> MAGSREILLPEVHLNSPIVKHKLYYYILLGNLPNEIDLDDLGPLHNQNWNQIAHEESNLAQRLVNVRNFLITHIPDLRKGHWQEYVNVILWPRILPLIPDFKINDQLPLLKNWDKLVKESCSVINAGTSQCIQNLSYGLTGRGNLFTRSRELSGDRRDIDLKTVVAAWHDSDWKRISDFWIMIKFQMRQLIVRQTDHNDSDLITYIENREGIIIITPELVALFNTENHTLTYMTFEIVLMVSDMYEGRHNILSLCTVSTYLNPLKKRITYLLSLVDNLAFQIGDAVYNIIALLESFVYAQLQMSDPIPELRGQFHAFVCSEILDALRGTNSFTQDELRTVTTNLISPFQDLTPDLTAELLCIMRLWGHPMLTASQAAGKVRESMCAGKVLDFPTIMKTLAFFHTILINGYRRKHHGVWPPLNLPGNASKGLTELMNDNTEISYEFTLKHWKEVSLIKFKKCFDADAGEELS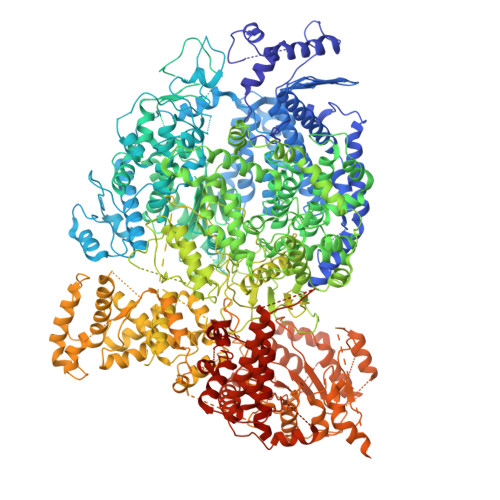IFMKDKAISAPKQDWMSVFRRSLIKQRHQHHQVPLPNPFNRRLLLNFLGDDKFDPNVELQYVTSGEYLHDDTFCASYSLKEKEIKPDGRIFAKLTKRMRSCQVIAESLLANHAGKLMKENGVVMNQLSLTKSLLTMSQIGIISEKARKSTRDNINQPGFQNIQRNKSHHSKQVNQRDPSDDFELAASFLTTDLKKYCLQWRYQTIIPFAQSLNRMYGYPHLFEWIHLRLMRSTLYVGDPFNPPADTSQFDLDKVINGDIFIVSPRGGIEGLCQKAWTMISIAVIILSATESGTRVMSMVQGDNQAIAVTTRVPRSLPTLEKKTIAFRSCNLFFERLKCNNFGLGHHLKEQETIISSHFFVYSKRIFYQGRILTQALKNASKLCLTADVLGECTQSSCSNLATTVMRLTENGVEKDICFYLNIYMTIKQLSYDIIFPQVSIPGDQITLEYINNPHLVSRLALLPSQLGGLNYLSCSRLFNRNIGDPVVSAVADLKRLIKSGCMDYWILYNLLGRKPGNGSWATLAADPYSINIEYQYPPTTALKRHTQQALMELSTNPMLRGIFSDNAQAEENNLARFLLDREVIFPRVAHIIIEQTSVGRRKQIQGYLDSTRSIMRKSLEIKPLSNRKLNEILDYNINYLAYNLALLKNAIEPPTYLKAMTLETCSIDIARNLRKLSWAPLLGGRNLEGLETPDPIEITAGALIVGSGYCEQCAAGDNRFTWFFLPSGIEIGGDPRDNPPIRVPYIGSRTDERRVASMAYIRGASSSLKAVLRLAGVYIWAFGDTLENWIDALDLSHTRVNITLEQLQSLTPLPTSANLTHRLDDGTTTLKFTPASSYTFSSFTHISNDEQYLTINDKTADSNIIYQQLMITGLGILETWNNPPINRTFEESTLHLHTGASCCVRPVDSCILSEALTVKPHITVPYSNKFVFDEDPLSEYETAKLESLSFQAQLGNIDAVDMTGKLTLLSQFTARQIINAITGLDESVSLTNDAIVASDYVSNWISECMYTKLDELFMYCGWELLLELSYQMYYLRVVGWSNIVDYSYMILRRIPGAALNNLASTLSHPKLFRRAINLDIVAPLNAPHFASLDYIKMSVDAILWGCKRVINVLSNGGDLELVVTSEDSLILSDRSMNLIARKLTLLSLIHHNGLELPKIKGFSPDEKCFALTEFLRKVVNSGLSSIENLSNFMYNVENPRLAAFASNNYYLTRKLLNSIRDTESGQVAVTSYYESLEYIDSLKLTPHVPGTSCIEDDSLCTNDYIIWIIESNANLEKYPIPNSPEDDSNFHNFKLNAPSHHTLRPLGLSSTAWYKGISCCRYLERLKLPQGDHLYIAEGSGASMTIIEYLFPGRKIYYNSLFSSGDNPPQRNYAPMPTQFIESVPYKLWQAHTDQYPEIFEDFIPLWNGNAAMTDIGMTACVEFIINRVGPRTCSLVHVDLESSASLNQQCLSKPIINAIITATTVLCPHGVLILKYSWLPFTRFSTLITFLWCYFERITVLRSTYSDPANHEVYLICILANNFAFQTVSQATGMAMTLTDQGFTLISPERINQYWDGHLKQERIVAEAIDKVVLGENALFNSSDNELILKCGGTPNARNLIDIEPVATFIEFEQLICTMLTTHLKEIIDITRSGTQDYESLLLTPYNLGLLGKISTIVRLLTERILNHTIRNWLILPPSLRMIVKQDLEFGIFRITSILNSDRFLKLSPNRKYLIAQLTAGYIRKLIEGDCNIDLTRPIQKQIWKALGCVVYCHDPMDQRESTEFIDININEEIDRGIDGEEI> M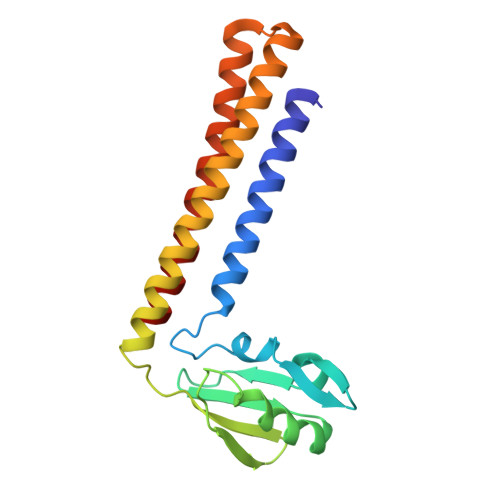TLKELYAETRSHMQKSLEVLEHNLAGLRTGRANPALLLHLKVEYYGAHVPLNQIATVTAPDPRTLVVQSWDQNALKAIEKAIRDSDLGLNPSNKGDALYINIPPLTEERRKDLVRAVRQYAEEGRVAIRNIRREALDKLKKLAKELHLSEDETKRAEAEIQKITDEFIAKADQLAEKKEQEILG> GPGGSGQGKSAREAAASLSLTLQKEGVIGVTEEQVHHIVKQALQRYSEDR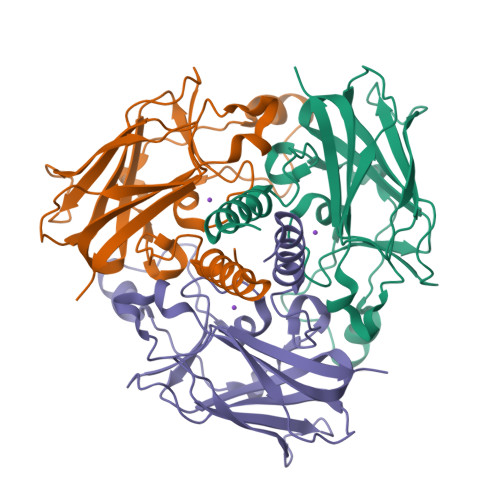IGLADYALESGGASVISTRCSETYETKTALLSLFGIPLWYHSQSPRVILQPDVHPGNCWAFQGPQGFAVVRLSARIRPTAVTLEHVPKALSPNSTISSAPKDFAIFGFDEDLQQEGTLLGKFTYDQDGEPIQTFHFQAPTMATYQVVELRILTNWGHPEYTCIYRFRVHGEPAH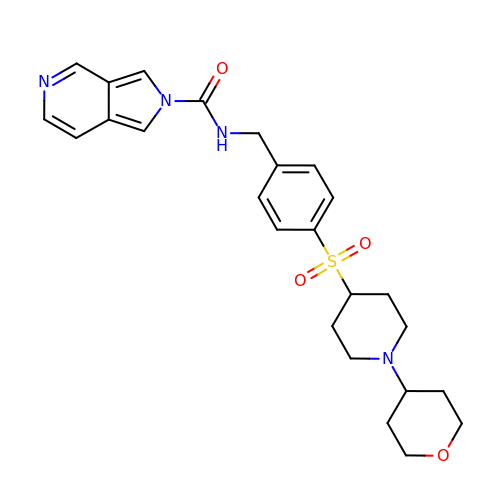N-(4-{[1-(tetrahydro-2H-pyran-4-yl)piperidin-4-yl]sulfonyl}benzyl)-2H-pyrrolo[3,4-c]pyridine-2-carboxamide | C25 H30 N4 O4 S | MQRGBJFQXJYKOD-UHFFFAOYSA-N> MSETQSQTMTRPQDLSLSDINSTVEVPEGHSFWKTLLAYSGPGALVAVGYMDPGNWSTSITGGQNFQYLLLSIIVISSLLAMLLQNMAAKLGIVCQLDLAQAIRARTSRRLGFIFWILTELAIMATDIAEVIGAAIALYLLFKIPIFLAVVITVLDVFLLLLLNRIGFRKIEALVVCLIFVILFVFLYQIILSQPAWHQVAKGLIPSWASVQTSPKIGGQTPLSASLGIIGATIMPANLFLHSAISQSRKIDR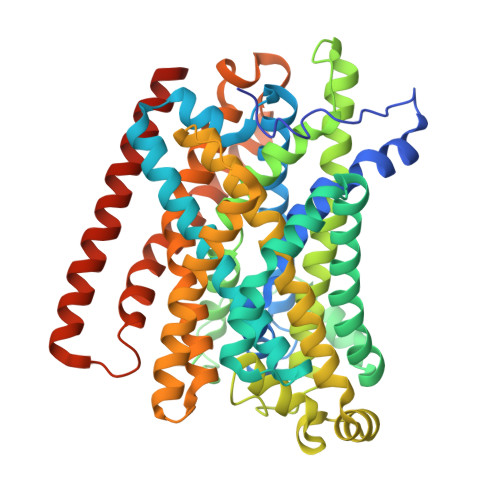TDSSKVAEAVRFSNWDSNIQLSLAMVVNALLLIMGVAVFKSGAVQDPSFFGLYQALSNPDMVSNPVLAEAARSGVLSTLFAVALLASGQNSTITGTITGQVIMEGFIHLRLPLWLRRLVTRLIAIIPVVVCVAITSHQGSLDEHQALNNLMNNSQVFLALALPFSIVPLLMLTDSAAQMGNQFKNTRWVKVMGWLTVIILTLLNLISISSQIAGFFGDNPSSQDLLLSQVISIGIILAMIGLLIWTIIDIRRFTHPKQKALEVLFQ Here, we have determined the structure and molecular architecture of the Ty3 capsid by 3D and 2D cryo-electron microscopy (cryo-EM) and compared it with those of the retroviruses. In the case of Ty3, Gag3 is cleaved into CA and NC domains. Formation of the capsid is important for genome protection and is an essential step in the retroelement life cycle. Similar to retroviruses, the protruding capsomers of the Ty3 capsid are formed by the CA-NTD, while the inner layer, linking the capsomers together, is formed by the CA-CTD.

To study the structure of PR- Ty3 particles at higher resolution, we collected a 2D cryo-EM dataset of the purified particles, identified the icosahedral particles by image classification, and determined their structure to 7.5-Å resolution using the RELION single-particle processing pipeline. The particles have a radius to the center of the CA layer of ∼24 nm. The location of pentamers confirmed the T = 9 symmetry identified by cryo-ET and subtomogram averaging. The reconstruction showed clear α-helical densities consistent with the determined resolution, as well as a disordered internal layer, which may correspond to NC and associated nucleic acid. Consistent with the principles of virus architecture described by Caspar and Klug, the T = 9 Ty3 particle capsid is formed from 540 copies of CA. There are nine different (non–symmetry-related) copies of CA (one in the fivefold, two in the threefold, and six in the pseudothreefold positions within the complete Ty3 particle). Comparing the nine different non–symmetry-related positions, the fold of the individual CA-NTDs and CA-CTDs does not change, but their relative orientations change. Notably, the trimeric appearance of the sixfold coordinated positions in the EM map is a result of adjacent CA-NTDs existing in two very different orientations [Fig. 3A, orientation A (cyan) and orientation B (dark blue)]. To generate a structural model for the complete PR- Ty3 capsid, we placed the models for the Ty3 CA-NTD and CA-CTD from flexible fitting back into all nine independent positions within the complete EM map and modeled the linker connecting the CA-NTD and the CA-CTD independently for all nine copies using Modeler. To assess the conformational variability of CA within the capsid, we superimposed and compared the nine independent copies of CA, showing large relative movements of the domains about the flexible interdomain linker.

>MSFMDQIPGGGNYPKLPVECLPNFPIQPSLTFRGRNDSHKLKNFISEIMLNMSMISWPNDASRIVYCRRHLLNPAAQWANDFVQEQGILEITFDTFIQGLYQHFYKPPDINKIFNAITQLSEAKLGIERLNQRFRKIWDRMPPDFMTEKAAIMTYTRLLTKETYNIVRMHKPETLKDAMEEAYQTTALTERFFPGFELDADGDTIIGATTHLQEEYDSDYDSEDNLTQNRYVHTVRTRRSYNKPMSNHRNRRNNNASREECIKNRLCFYCKKEGHRLNECRARKAVLTDLELESKDQQTLFIKTLPIVH[9x]>SLMADEIAKAQVARPGGDTIFGKIIRKEIPAKIIFEDDRCLAFHDISPQAPTHFLVIPKKHISQISVAEDDDESLLGHLMIVGKKCAADLGLNKGYRMVVNEGSDGGQSVYHVHLAVLGGRQMHWPPG[2x]

Diadenosine-5′,5-P1,P4-tetraphosphate (Ap4A) is a ubiquitous second messenger from bacteria to higher eukaryotes, which responds to environmental stresses and cell cycle phases. Ap4A then binds to the histidine triad nucleotide-binding protein 1 (HINT1), thereby disrupting the protein–protein interaction with microphthalmia-associated transcription factor (MITF), and the released MITF eventually promotes the transcription of mast cell activation genes. The HINT1 protein is a compact and symmetric dimer, with two adenosine pockets at opposite sides. Here we report that Ap4A specifically polymerizes HINT1 into (HINT1-Ap4A)n (HAn) filaments in solution and in the activated RBL cells.

We then made an H114A mutant to inactivate the hydrolysis activity of HINT1. We also solved the HINT1H114A-Ap5A structure in a similar crystal packing state as HINT1H114A-Ap4A. The five-phosphate linkage in Ap5A adopted a bent and zigzag conformation compared with the straight conformation of Ap4A, suggesting that the increased length of Ap5A is too long to stabilize the HAn interface as Ap4A does. The negative stain EM also showed little effect of Ap3A, Ap5A, or AMP to induce HINT1 filament compared with Ap4A. Therefore, Ap3A and Ap5A are not able to polymerize HINT1.>MKLKQVAD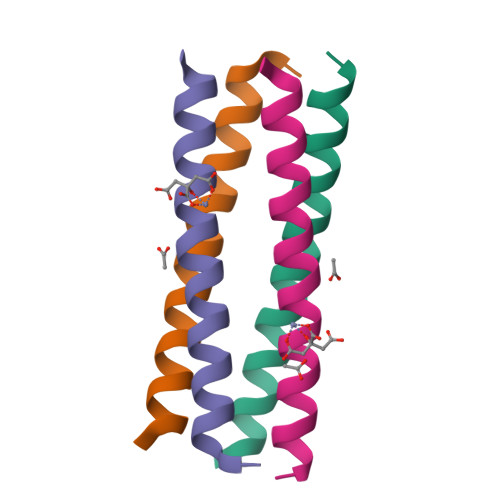KLEEVASKLYHNANELARVAKLLGER[8x]>[3x]MVVIANAHNELIHDAVLDYYGKRLATCSSDKTIKIFEVEGETHKLIDTLTGHEGPVWRVDWAHPKFGTILASCSYDGKVLIWKEENGRWSQIAVHAVHSASVNSVQWAPHEYGPLLLVASSDGKVSVVEFKENGTTSPIIIDAHAIGVNSASWAPATIEEDGEHNGTKESRKFVTGGADNLVKIWKYNSDAQTYVLESTLEGHSDWVRDVAWSPTVLLRSYLASVSQDRTCIIWTQDNEQGPWKKTLLKEEKFPDVLWRASWSLSGNVLALSGGDNKVTLWKENLEGKWEPAGEVHQ;>[3x]MGSSHHHHHHSQDPFSECNDEIDNAKLIMKERRFTASYTFAKFSTGSMLLTKDIVGKSGVSIKRLPTELQRKFLFDDVYLDKEIEKVTIEARKSNPYPQISESSLLFKDALDYMEKTSSDYNLWKLSSILFDPVSYPYKTDNDQVKMALLKKERHCRLTSWIVSQIGPEIEEKIRNSSNEIEQIFLYLLLNDVVRASKLAIESKNGHLSVLISYLGSNDPRIRDLAELQLQKWSTGGCSIDKNISKIYKLLSGSPFEGLFSLKELESEFSWLCLLNLTLCYGQIDEYSLESLVQSHLDKFSLPYDDPIGVIFQLYAANENTEKLYKEVRQRTNALDVQFCWYLIQTLRFNGTRVFSKETSDEATFAFAAQLEFAQLHGHSLFVSCFLNDDKAAEDTIKRLVMREITLLRASTNDHILNRLKIPSQLIFNAQALKDRYEGNYL;>MELSPTYQTERFTKFSDTLKEFKIEQNNEQNPIDPFNIIREFRSAAGQLALDLANSGDESNVISS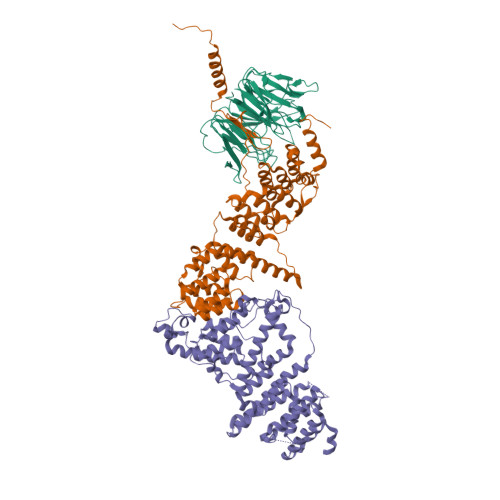KDWELEARFWHLVELLLVFRNADLDLDEMELHPYNSRGLFEKKLMQDNKQLYQIWIVMVWLKENTYVMERPKNVPTSKWLNSITSGGLKSCDLDFPLRENTNVLDVKDKEEDHIFFKYIYELILAGAIDEALEEAKLSDNISICMILCGIQEYLNPVIDTQIANEFNTQQGIKKHSLWRRTVYSLSQQAGLDPYERAIYSYLSGAIPNQEVLQYSDWESDLHIHLNQILQTEIENYLLENNQVGTDELILPLPSHALTVQEVLNRVASRHPSESEHPIRVLMASVILDSLPSVIHSSVEMLLDVVKGTEASNDIIDKPYLLRIVTHLAICLDIINPGSVEEVDKSKLITTYISLLKLQGLYENIPIYATFLNESDCLEACSFILSSLEDPQVRKK[3x]Protoglobin (Pgb) is a recently discovered haem-protein with distinct structural and functional features that make it unique within the globin superfamily. The MaPgb* structure can be considered as an expanded version of the 3/3 helical sandwich typical of “classical” globins (i.e. Mb), with an additional N-terminal extension, built by a 20-residue loop, followed by the Z-helix, which precedes the globin-fold conserved A-helix. Residues belonging to the Z-helix contribute to formation of the Pgb homodimer, which is centered on the intermolecular four-helix bundle built by the G- and H-helices of the two subunits. Thus, in Pgb the access of diatomic ligands, such as O2, CO, and NO, to the haem is granted by two orthogonal apolar tunnels that reach the haem distal region from entry sites at the B/G and B/E helix interfaces.

The sites of MaPgb*(III) mutations (Trp(60)B9Ala, Tyr(61)B10Ala, Phe(93)E11Leu, Leu(142)G4Ala, and Ile(149)G11Phe) are located in the surroundings of the haem, or along the two tunnels; the mutations were designed to evaluate the (structural) impact of the selected residues on the stabilization of the haem-Fe(III)-bound ligand and on the reshaping of the haem distal cavity/tunnel system. The other two mutations considered, Leu(142)G4Ala, localized at the proximal site just on top of His(120)F8, and Ile(149)G11Phe, adjacent to Trp(60)B9 in tunnel 1, do not produce any significant deviation in the overall conformation of the distal site and in the cyanide binding mode relative to the MaPgb*(III)-cyanide structure. off for cyanide dissociation from cyanide-bound MaPgb*(III) and Leu(142)G4Ala and from the Ile(149)G11Phe ferric mutants, all characterized by ligand stabilization through two H-bonds (to Trp(60)B9 and Tyr(61)B10), are lower than those reported for ligand dissociation from the Tyr(61)B10Ala and Trp(60)B9Ala MaPgb*(III)-cyanide species, characterized by ligand stabilization through one H-bond. Overall, the single mutations do not affect significantly the tertiary structure of the mutated proteins, which are always closely similar in their backbone to that of MaPgb*(III)-cyanide, displaying rms deviation values which range between 0.17 Å and 0.49 Å, calculated for 190 Cα atom pairs.

>MSVEKIPGYTYGETENRAPFNLEDLKLLKEAVMFTAEDEEYIQKAGEVLEDQVEEILDTWYGFVGSHPHLLYYFTSPDGTPNEKYLAAVRKRFSRWILDTSNRSYDQAWLDYQYEIGLRHHRTKKNQTDNVESVPNIGYRYAVAFIYPITATMKPFLARKGHTPEEVEKMYQAWFKATTLQVALWSYPYVKYGDF[2x]>MSASKMAMSNLEKILELVPLSPTSFVTKYLPAAPVGSKGTFGGTLVSQSLLASLHTVPLNFFPTSLHSYFIKGGDPRTKIT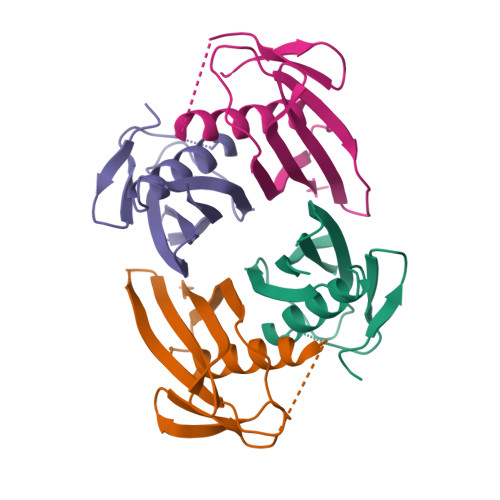YHVQNLRNGRNFIHKQVSAYQHDKLIFTSMILFAVQR[4x]> MSTSTEKRSKENLPWVEKYRPETLDEVYGQNEVITTVRKFVDEGKLPHLLFYGPPGTGKTSTIVALAREIYGKNYSNMVLELNASDDRGIDVVRNQIKDFASTRQIFSKGFKLIILDEADAMTNAAQNALRRVIERYTKNTRFCVLANYAHKLTPALLSRCTRFRFQPLPQEAIERRIANVLVHEKLKLSPNAEKALIELSNGDMRRVLNVLQSCKATLDNPDEDEISDDVIYECCGAPRPSDLKAVLKSILEDDWGTAHYTLNKVRSAKGLALIDLIEGIVKILEDYELQNEETRVHLLTKLADIEYSISKGGNDQIQGSAVIG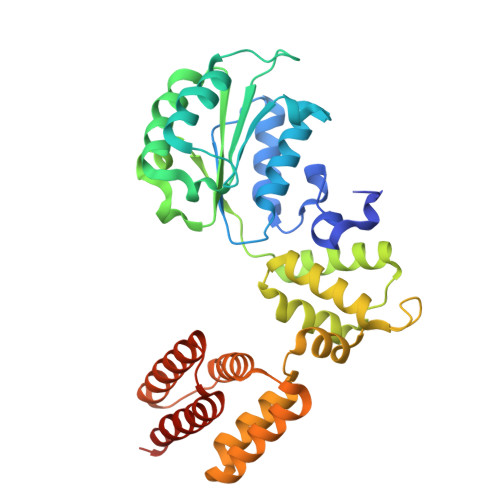AIKASFENETKANV> EERNDWHFNIGAMYEIENVEGYGEDMDGLAEPSVYFNAANGPWRIALAYYQEGPVDYSAGKRGTWFDRPELEVHYQFLENDDFSFGLTGGFRNYGYH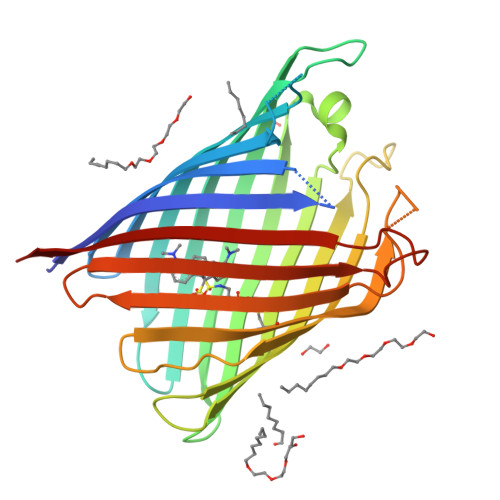YVDEPGKDTANMQRWKIAPDWDVKLTDDLRFNGWLSMYKFANDLNTTGYADTRVETETGLQYTFNETVALRVNYYLERGFNMDDSRNNGEFSTQEIRAYLPLTLGNHSVTPCTRIGLDRWSNWDWQDDIEREGHDFNRVGLFYGYDFQNGLSVSLEYAFEWQDHDEGDSDKFHYAGVGVNYSFHHHHHH> SLHMSFETRFEKMDNLLRDPKSEVNSDCLLDGLDALVYDLDFPALRKNKNIDNFLSRYKDTINKIRDLRMKAEDYEVVKVIGRGAFGEVQLVRHKSTRKVYAMKLLSKFEMIKRSDSAFFWEERDIMAFANSPWVVQLFYAFQDDRYLYMVMEYMPGGDLVNLMSNYDVPEKWARFYTAEVVLALDAIHSMGFIHRDVKPDNMLLDKSGHLKLADFGTCMKMNKEGMVRCDTAVGTPDYISPEVLKSQGGDGY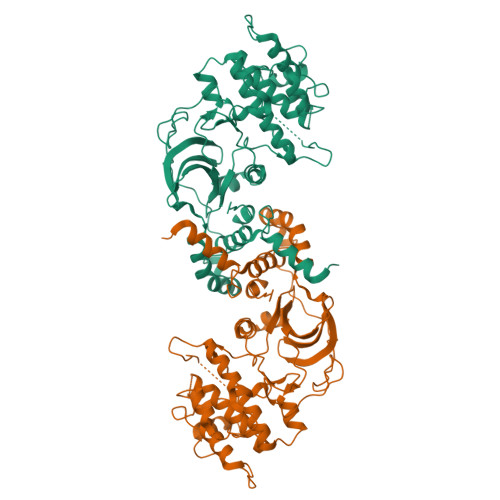YGRECDWWSVGVFLYEMLVGDTPFYADSLVGTYSKIMNHKNSLTFPDDNDISKEAKNLICAFLTDREVRLGRNGVEEIKRHLFFKNDQWAWETLRDTVAPVVPDLSSDIDTSNFDDLEEDKGEEETFPIPKAFVGNQLPFVGFTYYSNRRYLSSANPNDNR>[8x]MSLKITGVNIYLLKSGRLHPVLVEISTDEGITGAGEAGIAYGVGGTAAAGMIKDLSERFLIGKDPSRIEELWSTMYDHSFWAKNGGAIIFAGISAIEQALWDIKGKCLGVPVYELFGGKIRDRVRAYANGWYGAADTPDEFARAVERPLKEGYGALKFYPLAQRVGSALQHVTRRSMSAEAIELAYRRVKAVRDAAGPE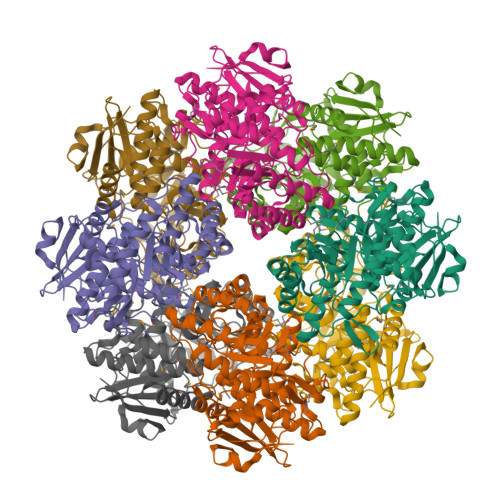IELMVDLSGGLTTDETIRFCRKIGELDICFVEEPCDPFDNGALKVISEQIPLPIAVGERVYTRFGFRKIFELQACGIIQPDIGTAGGLMETKKICAMAEAYNMRVAPHVCGSSLIETATLQLEANITNFMIHEHYPAFKADDGYVEVLENPPSISSGYFEMPNGPGLGAVLIKRNIEPYLWASCTEGHHHHHH>[2x]DLSPTSLREAFGHFPSGVIAIAAEVDGTRVGLAASTFVPVSLEPPLVAFAVQNSSTTWP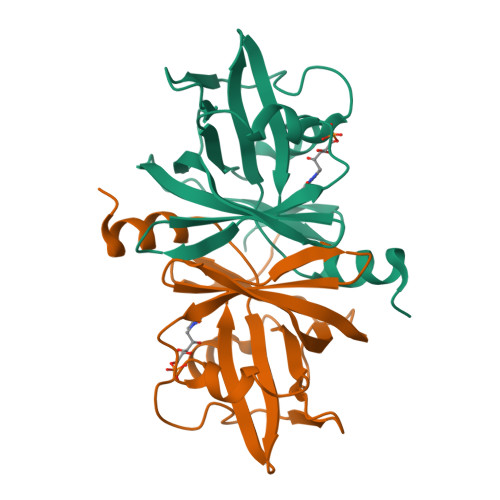KLKDLPSLGISVLGEAHDTAARTLAAKTGDRFAGLETESRDSGAVFINGTSVWLESAIEQLVPAGDHTIVVLRVSDIVINEAVPPIVFHRSAFRKLGA>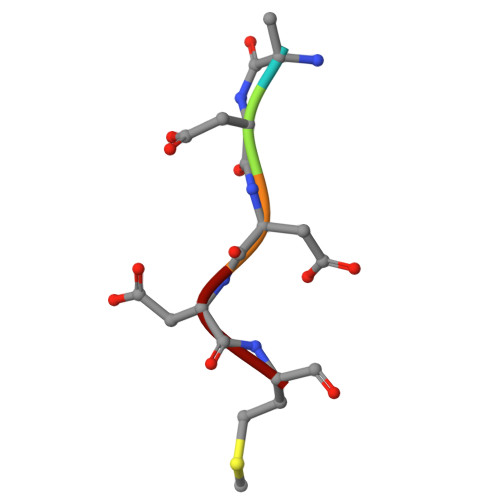 VDDDM> GATESGKRMDCPALPPGWKKEEVIRKSGLSAGKSE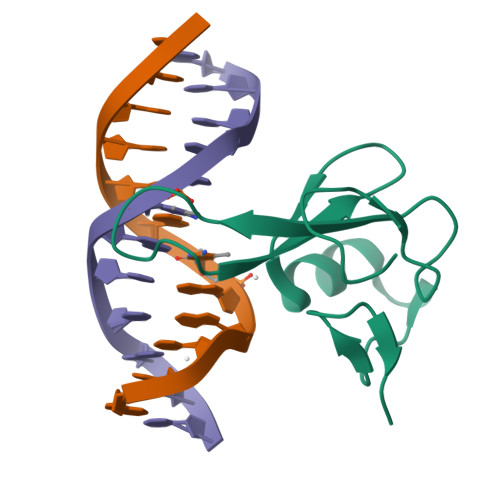VYYFSPSGKKFRSKPQLARYLGNTVDLSSFDFRTGKMMPSKLQK> LKGCWTKSIPPKPCF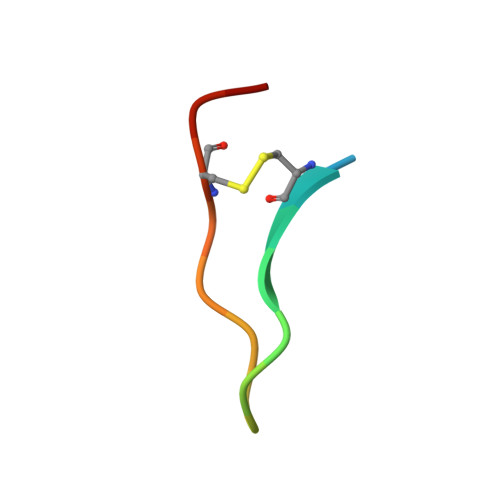GK2-(1-methylethyl)phenol | C9 H12 O | 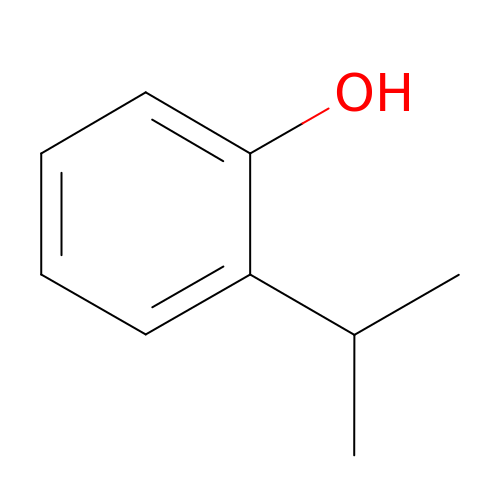CRBJBYGJVIBWIY-UHFFFAOYSA-N> QLNPYLRLKVRRDHIIDDALVRLEMIAMENPADLKKQLYVEFEGEQGVDEGGVSKEFFQLVVEEIFNPDIGMFTYD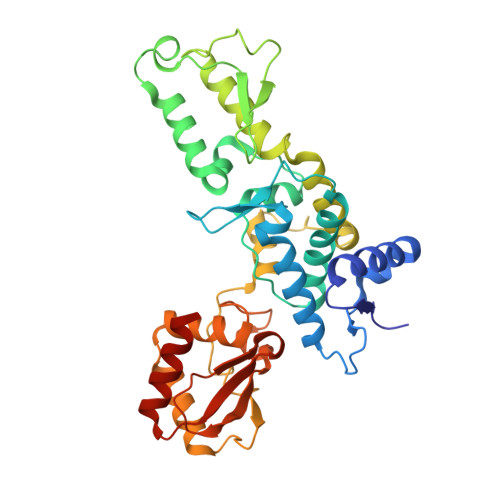ESTKLFWFNPSSFETEGQFTLIGIVLGLAIYNNCILDVHFPMVVYRKLMGKKGTFRDLGDSHPVLYQSLKDLLEYEGNVEDDMMITFQISQTDLFGNPMMYDLKENGDKIPITNENRKEFVNLYSDYILNKSVEKQFKAFRRGFHMVTNESPLKYLFRPEEIELLICGSRNLDFQALEETTEYDGGYTRDSVLIREFWEIVHSFTDEQKRLFLQFTTGTDRAPVGGLGKLKMIIAKNGPDTERLPTSHTCFNVLLLPEYSSKEKLKERLLKAITYAKGFGML> GSEFSLVAELQEKLQEEKAKFLEQLEEQEKRKNEEMQNVRTSLIAEQQTNFNTV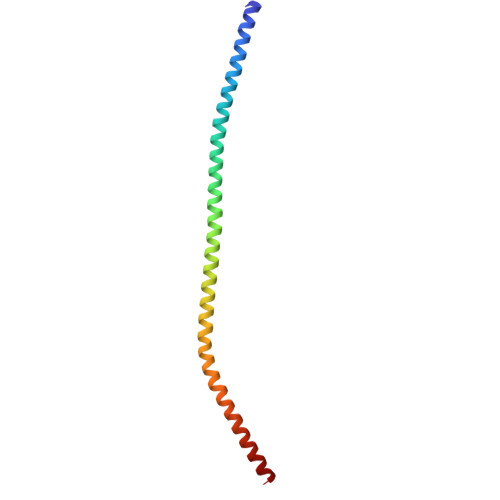LTREKMRKENIINDLSDKLKSTMQQQERDKDLIESLSEDRARLLEEKKKLEEEVSKLRSS Herein we have identified eight Sus-like systems in B. thetaiotaomicron that share the feature of a homologous SusE-like factor encoded immediately downstream from the transporter/lipoprotein duo susC/D. Two SusE-like proteins from these systems, BT2857 and BT3158, were characterized by X-ray crystallography and BT2857 was further analyzed by small-angle X-ray scattering. The SusE-like proteins were found to be composed of a conserved three domain architecture: a partially disordered N-terminal domain that is predicted to be proximal to the membrane and structurally homologous to an FN3-like bundle, a middle β-sandwich domain, and a C-terminal domain homologous to family 32 carbohydrate-binding modules, that bind to galactose. However, functional analyses with BT2857 and BT3158 revealed that the SusE-like proteins exhibited galactosidase activity with para-nitrophenyl-β-D-galactopyranoside and α-(1,4)-lactose substrates, that has not been demonstrated for SusE proteins. Using a series of domain truncations of BT2857, the predominant β-D-galactosidase activity is suggested to be localized to the C-terminal DUF5126 domain that would be most distal from the outer membrane.

The BT2857C construct crystallized in the P21 space group with two molecules in the asymmetric unit, and high-quality diffraction data was processed to 1.42 Å resolution. The structure of BT2857C adopts a β-sandwich fold with extensive loop regions and high similarity to the equivalent domain of BT3158. Structures of the DUF5000 or Ec domains (BT2857C and BT3158E223–P440) were compared via the MatchMaker in Chimera using the Smith-Waterman algorithm, yielding a RMSD of 1.225 Å across C-alpha atoms, and a quality score of 0.768. There is also high structural similarity of CBM32 with BT2857 (2.015 Å RMSD), including a calcium binding site wherein the calcium is coordinated by the side chains of N250, E391, main chain carbonyl oxygens of Y247, R252, T390, and a water (BT2857 numbering). Intriguingly, crystallographic ethylene glycol (EDO) that was supplemented during crystallization and used as a cryoprotectant was found in an equivalent location in BT2857 and BT3158. However, there is a lack of residue conservation at this site with the exception of a conserved histidine, H265 (BT2857 and BT3158). Notably, while not sequence conserved, the single Ramachandran outlier in BT2857 is D304. D304 is structurally oriented close to a channel occupied by D256, H265, and Y241. In this channel there are three conserved crystallographic ethylene glycol molecules that are present in both molecules in the asymmetric unit and could suggest the position of carbohydrates for modeling purposes. This region is equivalent to the position for carbohydrate accommodation by CBM family 32.

>[2x]MELDKTKFREMYLQNDSRVDSYDGKMEYVWNGRISKDGDSGGVGLHTGTGTKDGPAVFTFDLGVLAKLSRFALWAIQDEKHFYNDMSPRRYEVWGCATEPNPDGSWDQWVKLLDMENVKPSGSPIGILTEDDIEAAKIGDQANVPLDMPRVRYIRIKCLKNWSNNYNICFTELTFWGND3-aminocyclohexa-1,3-diene-1-carboxylic acid | C7 H9 N O2 | 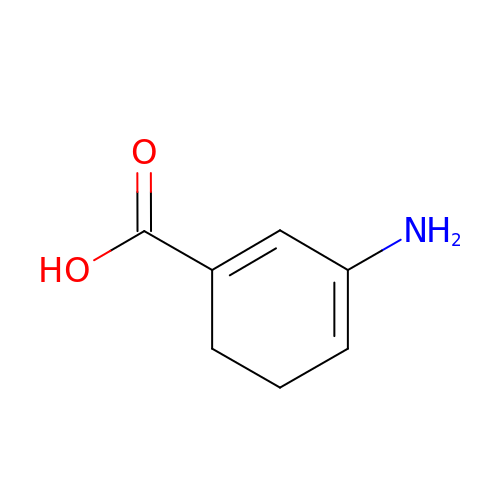CMKSBGMWHUXBKM-UHFFFAOYSA-N> ANIVGGIEYSINNASLCSVGFSVTRGATKGFVTAGHCGTVNATARIGGAVVGTFAARVFPGNDRAWVSLTSAQTLLPRVANGSSFVTVR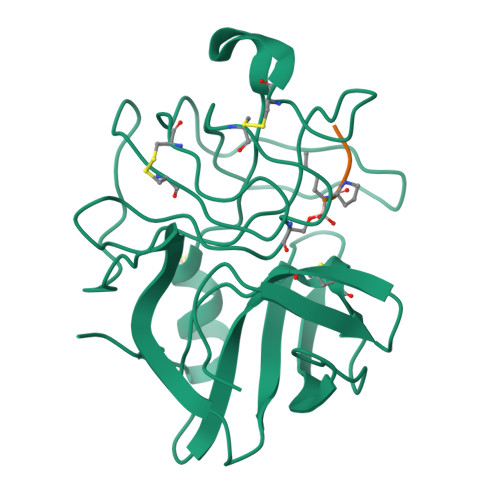GSTEAAVGAAVCRSGRTTGYQCGTITAKNVTANYAEGAVRGLTQGNACMGRGDSGGSWITSAGQAQGVASGGNVQSNGNNCGIPASQRSSLFERLQPILSQYGLSLVTG;> XAAPL> NQSKILTLQAYDPAKVLVFIGGQRVSGFAADTKIVITR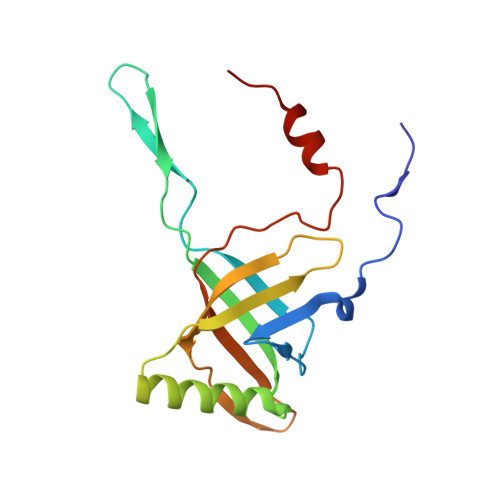NNDNISVHAGVDGEISNALSRDNTGVMTLSLQNTAKWNGYLAQWQRQANVTGLIYLPVQVEGSQGLSLNTIGWIQKQPDLSYGTEVGQMDWEIGVLDAWLSPDQIQGIAAGITGLLGL>TSHHGYQPFDMHNPFPAYKELRQEEPVMFDERIGYWVVTKYDDIKTTFDDWETFSSENAQAPVRKRGPQATQIMTDGGFTAYSGLS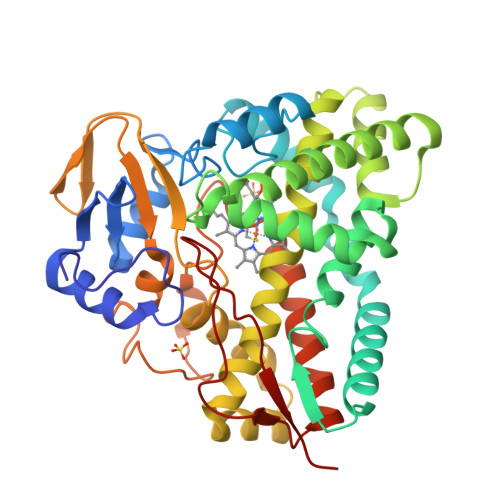ARIPPEHTRIRAIAQKAFTPRRYKALEPDIRAMVIDRVEKMLANDQHVGDMVSDLAYDIPTITILTLIGADISMVDTYKRWSDSRAAMTWGDLSDEEQIPHAHNLVEYWQECQRMVADAHAHGGDNLTADLVRAQQEGQEITDHEIASLLYSLLFAGHETTTTLISNCFRVLLDHPEQWQAILENPKLIPAAVDEVLRYSGSIVGWRRKALKDTEIGGVAIKEGDGVLLLMGSANRDEARFENGEEFDISRANAREHLSFGFGIHYCLGNMLAKLQAKICLEEVTRLVPSLHLVADKAIGFRENLSFRVPTSVPVTWNA[4x]>[2x]GHMNSFVGLRVVAKWSSNGYFYSGKITRDVGAGKYKLLFDDGYECDVLGKDILLCDPIPLDTEVTALSPNEYFSAGVVKGHRKESGELYYSIEKEGQRKWYKRMAVILSLEQGNRLREQYGLG

The DNA damage response protein 53BP1 (p53-binding protein 1) influences the cell cycle dependency of DNA double-strand break (DSB) repair pathway selection. The localization of 53BP1 to chromatin also requires that it binds histone H4 di-methylated at K20 (H4K20me2) via a tandem Tudor domain (53BP1TT), while BRCA1-BARD1 recruitment requires unmethylated H4K20 recognized by an Ankyrin repeat domain in BARD1. We show that a series of water-soluble small molecules targeting the methyl-lysine binding cavity in 53BP1TT function by stabilizing a previously unknown lowly populated autoinhibited homodimeric state of 53BP1TT in which the histone binding surface of H4K20me2 is buried within the protomeric interface. Our work therefore identifies an auto-associated form of 53BP1—autoinhibited for chromatin binding—that can be stabilized by small molecule ligands encapsulated between two 53BP1 protomers.

To test the possibility of a pre-existing 53BP1TT homodimer, we created a 53BP1TT mutant (53BP1TT-PN) in which E1549 and D1550 were replaced by a proline and an asparagine, respectively, to introduce a 3D structure-preserving β-turn in 53BP1TT. These mutations eliminate the six salt bridges at the 53BP1TT dimer interface but do not affect the small molecule-binding surface. We verified that the structural integrity of 53BP1TT-PN was preserved by determining a 2.20 Å resolution crystal structure of this protein variant. The backbone dynamic properties of wild-type 53BP1TT and 53BP1TT-PN were quite similar as shown using NMR relaxation measurements. As expected, 53BP1TT-PN also bound UNC1078. The most likely interpretation for the absence of interaction of 53BP1TT-PN with UNC2170, UNC2991 and UNC3474 is that these small molecules do not cause 53BP1TT dimerization directly. Instead, they only bind to and stabilize a pre-existing 53BP1TT homodimer population, shifting the equilibrium toward homodimer. When overlaid, the 1H-15N HSQC spectra of wild-type 53BP1TT and 53BP1TT-PN showed small chemical shift changes that map to the inter-53BP1TT interface in 53BP1TT-UNC3474. This is further evidence for a preexisting small population of 53BP1TT homodimer that is eliminated in 53BP1TT-PN. We showed that 53BP1TT constructs engineered to prevent auto-association—while preserving the ligand binding cage—have no affinity for the small molecule ligands, and yet, they bind H4KC20me2 and p53K382me2 like wild-type 53BP1TT.> MKRLTYISKFSRPLSGDEIEAIGRISSQKNQQANVTGVLLCLDGIFFQILEGEAEKIDRIYERILADERHTDILCLKSEVEVQERMFPDWSMQTINLDENTDFLIRPIKVLLQTLTESHRILEKYTQPSIFKIISQGTNPLNIRPKAVEKIVFFSDIVSFSTF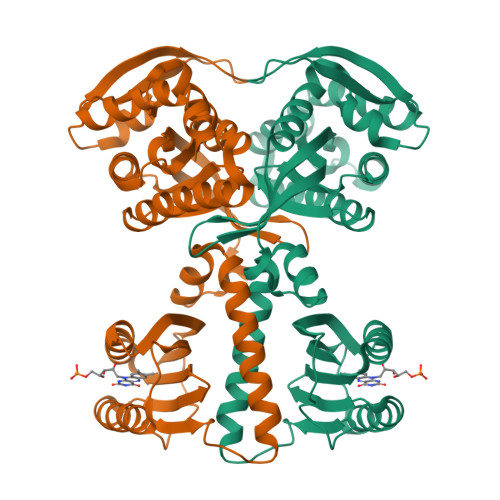AEKLPVEEVVSVVNSYFSVCTAIITRQGGEVTKFIGDCVMAYFDGDCADQAIQASLDILMELEILRNSAPEGSPLRVLYSGIGLAKGKVIEGNIGSELKRDYTILGDAVNVAARLEALTRQLSQALVFSSEVKNSATKSWNFIWLTDSELKGKSESIDIYSIDNEMTRKSSGGLEIARNIGHYLERV>[4x]SMALYRVVLLGDPGVGKTSLASLFAGKQERDLHEQLGEDVYERTLTVDGEDTTLVVVDTWEAEKLDKSWSQESC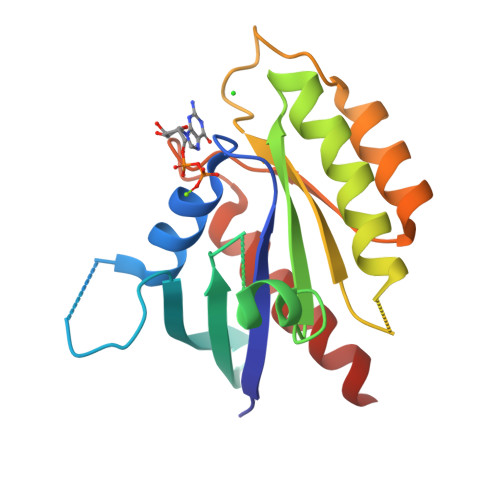LQGGSAYVIVYSIADRGSFESASELRIQLRRTHQADHVPIILVGNKADLARCREVSVEEGRACAVVFDCKFIETSATLQHNVAELFEGVVRQLRLRRRDSA>MSKDYQSLAKLSPFELKDELIKIASSDGNRLMLNAGRGNPNFLATTPRRAFFRLGLFAAAESELSYSYMTTVGVGGLAKIDGIEGRFERYIAENRDQEGVRFLGKSLSYVRDQLGLDPAAFLHEMVDGILGCNYPVPPRMLNISEKIVRQYIIREMGADAIPSESVNLFAVEGGTAAMAYIFESLKLNGLLKAGDKVAIGMPVFTPYIEIPELAQYALEEVAINADPSLNWQYPDSELDKLKDPAIKIFFCVNPSNPPSVKMDQRSLERVRNIVAEHRPDLMILTDDVYGTFADDFQSLFAICPENTLLVYSFSKYFGATGWRLGVVAAHQQNVFDLALDKLQESEKVALDHRYRSLLPDVRSLKFIDRLVADSRAVALNH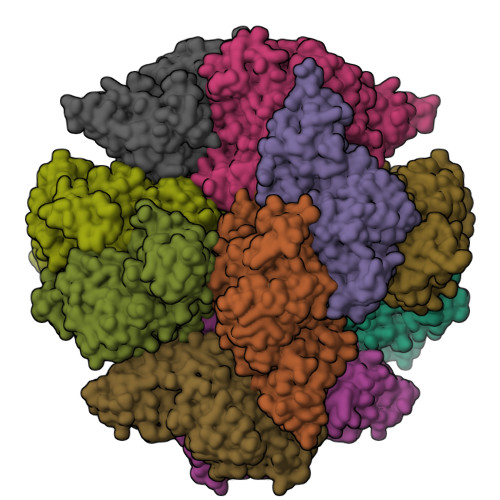TAGLSTPQQVQMALFSLFALMDEADEYKHTLKQLIRRRETTLYRELGMPPLRDENAVDYYTLIDLQDVTAKLYGEAFSEWAVKQSSTGDMLFRIADETGIVLLPGAGFGSNRPSGRASLANLNEYEYAAIGRALRKMADELYAEYSGQAQNLKLAAALEHHHHHH[6x]> MQSNKTFNLEKQNHTPRKHHQH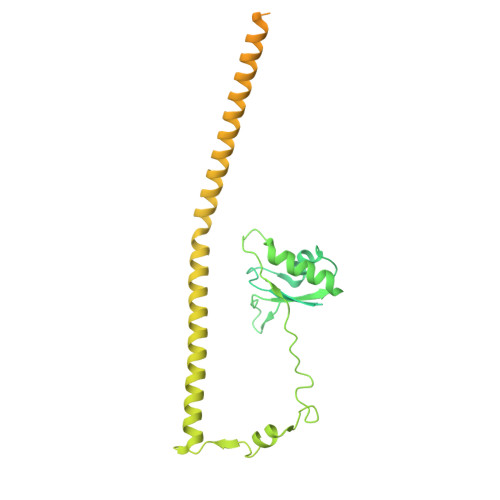HHQQHHQQQQQQQQQPPPPIPANGQQASSQNEGLTIDLKNFRKPGEKTFTQRSRLFVGNLPPDITEEEMRKLFEKYGKAGEVFIHKDKGFGFIRLETRTLAEIAKVELDNMPLRGKQLRVRFACHSASLTVRNLPQYVSNELLEEAFSVFGQVERAVVIVDDRGRPSGKGIVEFSGKPAARKALDRCSEGSFLLTTFPRPVTVEPMDQLDDEEGLPEKLVIKNQQFHKEREQPPRFAQPGSFEYEYAMRWKALIEMEKQQQDQVDRNIKEAREKLEMEMEAARHEHQVMLMRQDLMRRQEELRRMEELHNQEVQKRKQLELRQEEERRRREEEMRRQQEEMMRRQQEGFKGTFPDAREQEIRMGQMAMGGAMGINNRGAMPPAPVPTGTPAPPGPATMMPDGTLGLTPPTTERFGQAATMEGIGAIGGTPPAFNRPAPGADFAPNKRRRY>[4x]MRLEVFCEDRLGLTRELLDLLVLRGIDLRGIEIDPIGRIYLNFAELEFESFSSLMAEIRRIAGVTDVRTVPWMPSEREHLALSALLEALPEPVLSVD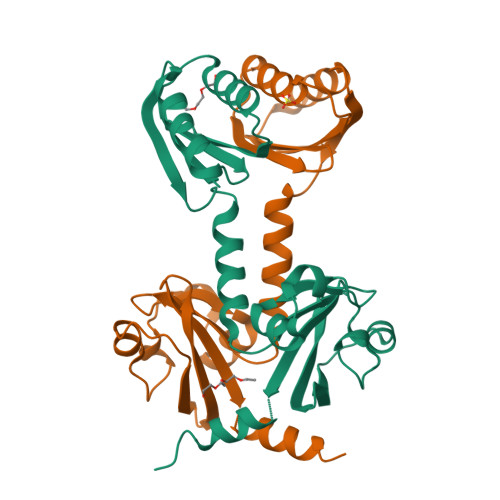MKSKVDMANPASCQLFGQKLDRLRNHTAAQLINGFNFLRWLESEPQDSHNEHVVINGQNFLMEITPVYLQDENDQHVLTGAVVMLRSTIRMGR>MLLNRANSTDSLSFSFINFDRDERNLIFQGDAHTSRNNILQLTRTDSNGAPVRSTVGRILHSAQVRLWEKSTNRVANLQTQFSFFLSSPLSNPADGIAFFIAPPDTTIPSGSAGGLLGLFNPRTALNESANQVLAVEFDTFFAQNSNT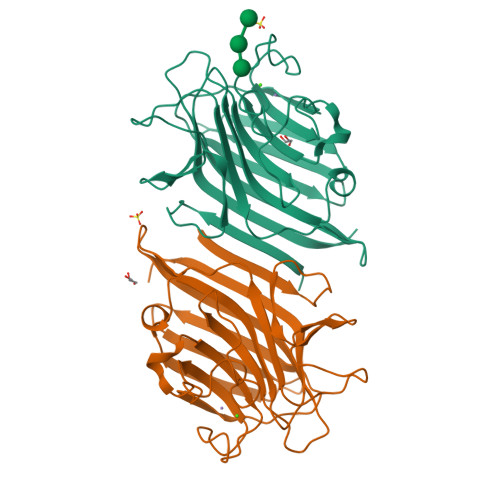WDPNYQHIGIDVNSIRSSKVVRWERREGKTLNVLVTYNPSTRTIDVVATYPDGQRYQLSHVVDLTTILPEWVRVGFSAASGEQFQTHNLESWSFTSTLLYTAQKEDEYLARDM[2x]> GPAQSGTLGGFSKPQKTFVRPGGGVGYKGKGVWTG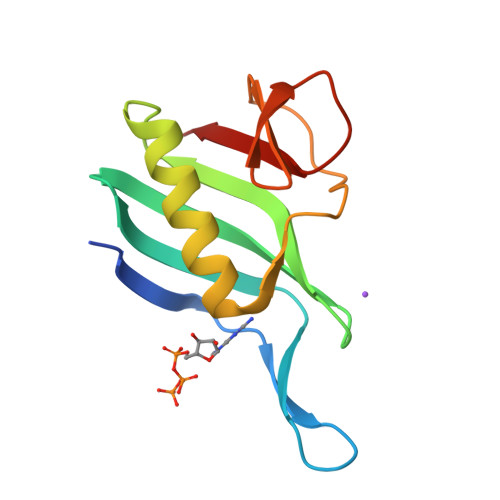VMEDTHVQILIDGDGTSNWLEEIRLSSDARLYDVIESIRRLCDDLGINNRVASAYRGHCMVRLSGFKIKPASRTDGCPVRIME> GPGYQDPLSIDERLQALVYRELNNAVAFNKAESGSAVLVDVNTGEVLAMANSPGRNRTITDVFEPGSTVKPMVVMTALQRGVVRENSVLNTIPYRINGHEIKDVARYSELTLTGVLQKSSNVGVSKLALAMPSSALV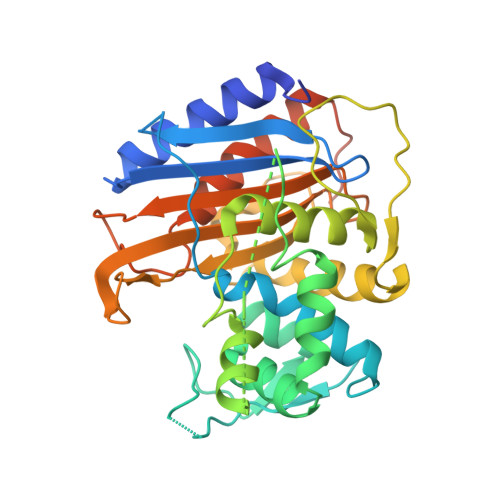DTYSRFGLGKATNLGLVGERSGLYPQKQRWSDIERATFSFGYGLMVTPLQLARVYATIGSYGIYRPLSITKVDPPVPGERVFPESIVRTVVHMMESVALPGGGGVKAAIKGYRIAIKTGTAKKVGPDGRYINKYIAYTAGVAPASQPRFALVVVINDPQAGKYYGGAVSAPVFGAIMGGVLRTMNIEPDALTTGDKNEFVINQGEGTGGRS> AKPLTDQEKRRQISIRGIVGVENVAELKKSFNRHLHFTLVKDRNVATTRDYYFALAHTVRDHLVGRWIRTQQHYYDKCPKRVYYLSLEFYMGRTLQNTMINLGLQNACDEAIYQLGLDIEELEEIEEDAGLGNGGLGRLAACFLDSMATLGLAAYGYGIRYEYGIFNQKIRDGWQVEEADDWLRYGNP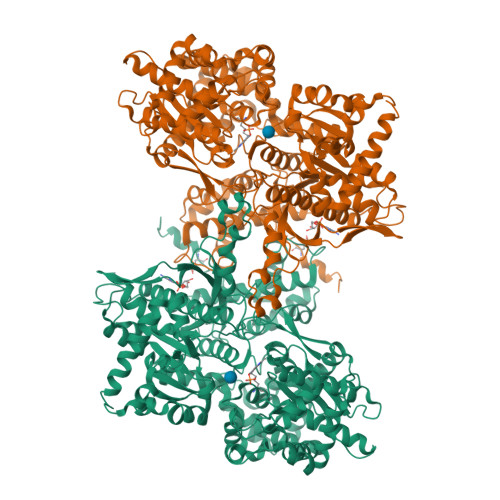WEKSRPEFMLPVHFYGKVEHTNTGTKWIDTQVVLALPYDTPVPGYMNNTVNTMRLWSARAPNDFNLRDFNVGDYIQAVLDRNLAENISRVLYPNDNFFEGKELRLKQEYFVVAATLQDIIRRFKASKFGSTRGAGTVFDAFPDQVAIQLNDTHPALAIPELMRIFVDIEKLPWSKAWELTQKTFAYTNHTVLPEALERWPVDLVEKLLPRHLEIIYEINQKHLDRIVALFPKDVDRLRRMSLIEEEGSKRINMAHLCIVGSHAVNGVAKIHSDIVKTKVFKDFSELEPDKFQNKTNGITPRRWLLLCNPGLAELIAEKIGEDYVKDLSQLTKLHSFLGDDVFLRELAKVKQENKLKFSQFLETEYKVKINPSSMFDVQVKRIHEYKRQLLNCLHVITMYNRIKKDPKKLFVPRTVIIGGKAAPGYHMAKMIIKLITSVADVVNNDPMVGSKLKVIFLENYRVSLAEKVIPATDLSEQISTAGTEASGTGNMKFMLNGALTIGTMDGANVEMAEEAGEENLFIFGMRIDDVAALDKKGYEAKEYYEALPELKLVIDQIDNGFFSPKQPDLFKDIINMLFYHDRFKVFADYEAYVKCQDKVSQLYMNPKAWNTMVLKNIAASGKFSSDRTIKEYAQNIWNVEPSDLKISLSNESNKVNGN IMP-type metallo-β-lactamases confer resistance to carbapenems and a broad spectrum of β-lactam antibiotics. IMP-6 and IMP-1 differ by only a point mutation: Ser262 in IMP-1 and Gly262 in IMP-6. The overall structures of IMP-6 and IMP-1 are similar.

Here, we report the crystal structures of IMP-6 and IMP-1 with the same space group and similar cell constants at resolutions of 1.70 and 1.94 Å, respectively. The kcat/Km values of IMP-1 for imipenem and meropenem are nearly identical; however, for IMP-6, the kcat/Km for meropenem is 7-fold that for imipenem. However, the loop region (residues 60–66), which participates in substrate binding, is more flexible in IMP-6 than in IMP-1. This difference in flexibility determines the substrate specificity of IMP-type metallo-β-lactamases for imipenem and meropenem. The amino acid at position 262 alters the mobility of His263; this affects the flexibility of the loop via a hydrogen bond with Pro68, which plays the role of a hinge in IMP-type metallo-β-lactamases. The substitution of Pro68 with a glycine elicited an increase in the Km of IMP-6 for imipenem, whereas the affinity for meropenem remained unchanged.

>MSKLSVFFIFLFCSIATAAESLPDLKIEKLDEGVYVHTSFEEVNGWGVVPKHGLVVLVNAEAYLIDTPFTAKDTEKLVTWFVERGYKIKGSISSHFHSDSTGGIEWLNSRSIPTYASELTNELLKKDGKVQATNSFSGVNYWLVKNKIEVFYPGPGHTPDNVVVWLPERKILFGGCFIKPYGLGNLGDANIEAWPKSAKLLKSKYGKAKLVVPGHSEVGDASLLKLTLEQAVKGLNESKKPSKPSN[4x]>[2x]MSKYKLIMLRHGEGAWNKENRFCSWVDQKLNSEGMEEARNCGKQLKALNFEFDLVFTSVLNRSIHTAWLILEELGQEWVPVESSWRLNERHYGALIGLNREQMALNHGEEQVRLWRRSYNVTPPPIEESHPYYQEIYNDRRY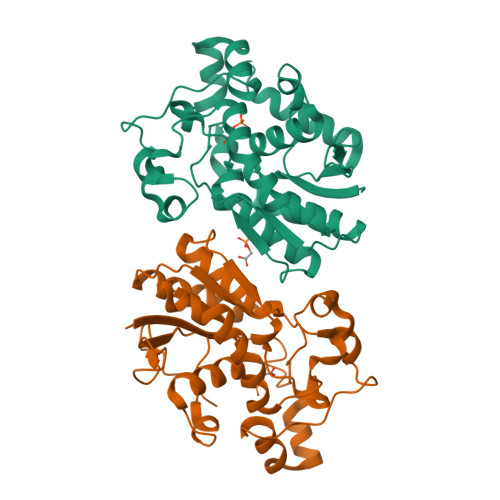KVCDVPLDQLPRSESLKDVLERLLPYWNERIAPEVLRGKTILISAHGNSSRALLKHLEGISDEDIINITLPTGVPILLELDENLRAVGPHQFLGDQEAIQAAIKKVEDQGKVKQAKKLEHHHHHH Spermidine synthase (SpdS; putrescine aminopropyltransferase) catalyzes the transfer of the aminopropyl moiety from decarboxylated S-adenosylmethionine to putrescine, leading to the formation of spermidine and 5′-methylthio­adenosine (MTA). In this work, X-ray crystallography was used to examine ligand complexes of SpdS from the malaria parasite Plasmodium falciparum (PfSpdS). The active site of SpdS is located between the domains and consists of two interconnected clefts for binding dcAdoMet and putrescine. A conserved flexible structural element called the gatekeeper loop covers the active site of the enzyme.

In the present study, X-ray crystal structures of PfSpdS were solved in complex with MTA and the substrate putrescine, and with the reaction products MTA and spermidine, which was obtained by soaking putrescine into crystals of PfSpdS in complex with dcAdoMet. When putrescine was soaked into crystals of the complex of PfSpdS with dcAdoMet the crystals were not visibly altered and diffraction data were collected to 1.75 Å resolution. The occupancy of the two ligands is 100% in all of the molecules in the asymmetric unit, suggesting that complete conversion occurs in the crystals. No changes were observed in residue conformations around MTA or spermidine compared with the structures containing either dcAdoMet or putrescine. This is consistent with the observed stability of the crystals upon addition of putrescine.

>GSKKWFSEFSIMWPGQAFSLKIKKILYETKSKYQNVLVFESTTYGKVLVLDGVIQLTEKDEFAYHEMMTHVPMTVSKEPKNVLVVGGGDGGIIRELCKYKSVENIDICEIDETVIEVSKIYFKNISCGYEDKRVNVFIEDASKFLENVTNTYDVIIVDSSDPIGPAETLFNQNFYEKIYNALKPNGYCVAQCESLWIHVGTIKNMIGYAKKLFKKVEYANISIPTYPCGCIGILCCSKTDTGLTKPNKKLESKEFADLKYYNYENHSAAFKLPAFLLKEIENI[3x]>MAGNFSEIESQGNISLKFGFLGLGMGGCAIAAECANKETQIKNNKYPYRAILVNTNSQDFNKIEIKNTGNVRKIQLEGYEQGAARNPQVGEEAFVKHETKIFEAVKQEFEDRDFIWITCGLGGGTGTGALLKAIEMLYEHDYNFGLLLTLPRDAEALKVLENATSRIRSIAMNQEAFGSIVLIDNAKLYRKFEEENPSALANEYTSYSNKYIADALHEINLVTSSFTPFSDTHFDASEFAQVINTPGVLSLAKLELKSNQLDTENPLGYLTQLG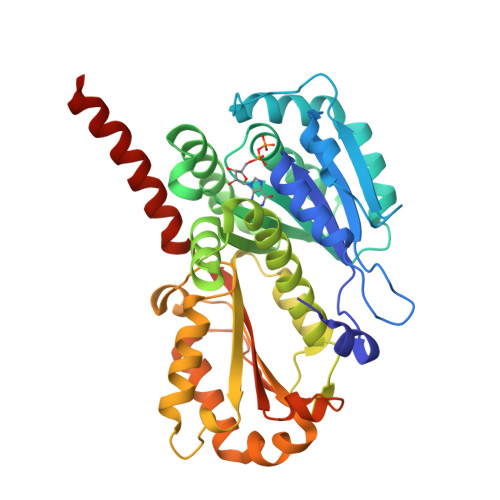NALEKGVLYDTEREELESAKKSALSIVTSPLRAGRLYNFSFLNQMENFLKERTPYVDERPIAPYVNKHTTKKEEDIVKFYSVVAGLPLPKRVSDIIDEITRIKEEREQANSKKSN[2x]Through an in silico approach to identify new macrodomain-containing proteins in this organism, we identify a protein containing regions of similarity to aprataxin, APLF and PNKP that we call APL (aprataxin/APLF-and-PNKP-like protein). Interestingly, the N- and C-termini of the APL macrodomain align with the C- and N-termini of human macrodomains, respectively, indicating it has undergone a circular permutation during evolution. In order to assess whether these permuted macrodomains retain important structural characteristics, we solved the X-ray crystal structures of the isolated permutated macrodomains found in Dictyostelium APL and O. sativa Q10MW4. Structural analysis of this novel macrodomain indicates it has retained the core features of this domain family, including the α-β-α sandwich fold consisting of a six-stranded β-sheet flanked by α-helices.

A BLAST database search with the macrodomain sequence of APL identifies the permuted macrodomain in a small number of other organisms, including the plants Arabidopsis thaliana and Oryza sativa. These permutated domains show a high level of primary sequence conservation with that found in APL, indicating that the same permuted macrodomain is present in several diverse species and implying that it is functionally important. Subsequently, X-ray data from the O. sativa macrodomain was solved through molecular replacement with PHASER by using the Dictyostelium macrodomain structure as the search model. We were able to obtain the O. sativa macrodomain in a complex with ADP-ribose, further confirming that the canonical mode of interaction with ADP-ribose is also retained. For example, the acidic amino acids D175 (E439 in Dictyostelium) that forms hydrogen bonds with the ADP-ribose ligand, and the aromatic F113 that forms the binding pocket for the distal ribose unit are found in O. sativa Q10MW4 and canonical macrodomains, suggesting that these amino acids will perform the same functions in most macrodomains. Additionally, F113, which forms a binding pocket for the distal ribose unit, is absolutely conserved, and the two substrate-binding loops (loops 1 and 2) that flank the pyrophosphate of the ADP-ribose are also apparent. Moreover, several key amino acids within the ADP-ribose-binding pocket that coordinate ADP-ribose binding are conserved in this domain. Of note, the APL macrodomain in plants is fused to two other DNA repair domains, aprataxin and polynucleotide kinase domains, strongly implying that APL supports DNA repair in plants as well.

>MGHHHHHHGGVKKELSNSKKIEDQSRESVLSDISSRTLAFPSISTADFQFDLDRASDIIVDAVADILQKYDNIRLVLVDLSHKSRILSLVKEKAAKKNINSSRFFTFVGDITQLQSKGGLRCNVIANAANWRLKPGGGGVNAAIYNAAGEDLQRATKECADTLRPGSSVAVPLPSTSPLHQREGVTHIIHVLGPNMNPMRPDCLKNDYTKGSKILHEAYTSLFENFVAIVQ[2x]(3R,4R)-3,4-dihydroxy-4-(hydroxymethyl)oxolan-2-one | C5 H8 O5 | 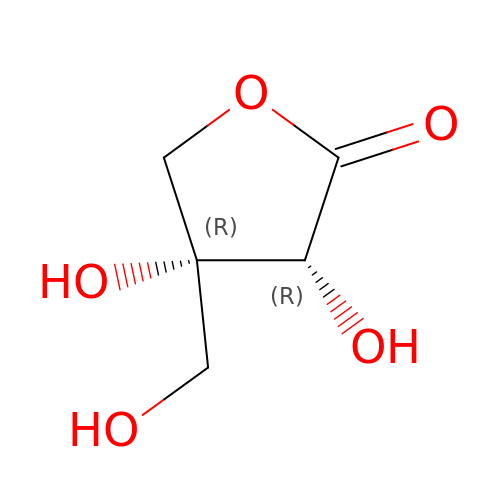MTSAHRPUAGVYCZ-WVZVXSGGSA-N6-(2-{3-[3-(dimethylamino)propyl]-2,5,6-trifluorophenyl}ethyl)-4-methylpyridin-2-amine 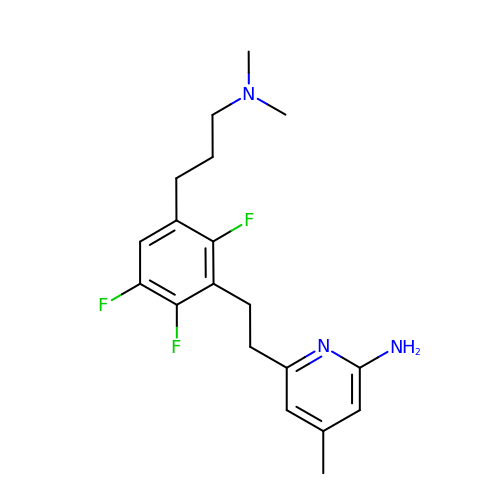| C19 H24 F3 N3 | ZAJCMGYRPZNQGR-UHFFFAOYSA-N> MKIGIIAAMPEELAYLVQHLDNAQEQVVLGNTYHTGTIVSHEVVLVESGIGKVMSAMSVAILAVHFQVDALINTGSAGAVAEGIAVGDVVIADKLAYHDVDVTAFGYAYGQMAQQPLYFESDKTFVAQIQESLSQLDQNWHLGLIATGDSFVAGNDKIEAIKSHFPEVLAVEMEGAAIAQAAHA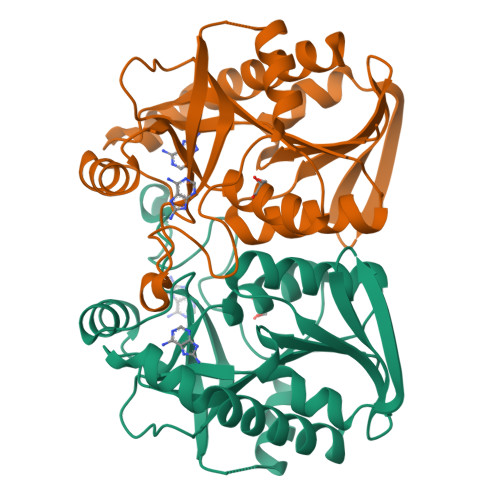LNLPVLVIRAMSDNANHEANIFFDEFIIEAGRRSAQVLLAFLKALD> MKELIYIEEPKILFAHGQKCTDARDGLALFGPLNNLYGIKSGVIGTKQGLKIFRDYLDHIQKPIYNSNSITRPMFPGFEAVFDCKWESTGITFKEVTNEDIGKFLYNSSTHKRTYDLVSLFIDKIISANKNEDENVDVWFVIVPDEIYKYCRPNSVLPKEMVQTKALMSKSKAKSFRYEPSLFPDI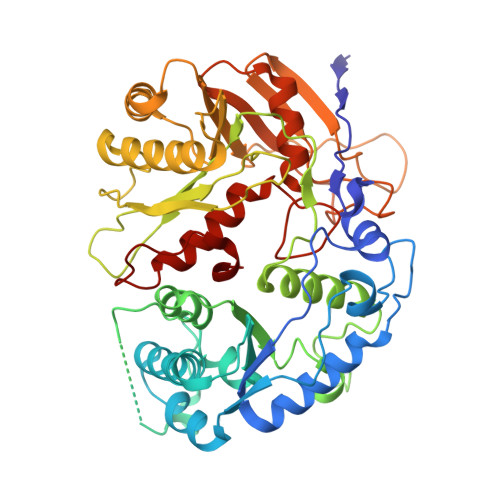NIELKEQEKEAETYNYDAQFHDQFKARLLKHTIPTQIFRESTLAWRDFKNAFGLPIRDFSKIEGHLAWTISTAAFYKAGGKPWKLSDVRNGVCYLGLVYKKVEKSKNPRNACCAAQMFLDNGDGTVFKGEVGPWYNPKNGQYHLEPKEAKALLSQSLQSYKEQIGEYPKEVFIHAKTRFNHQEWDAFLEVTPKETNLVGVTISKTKPLKLYKTEGDYTILRGNAYVVNERSAFLWTVGYVPKIQTALSMEVPNPLFIEINKGEADIKQVLKDILSLTKLNYNACIFADGEPVTLRFADKIGEILTASTDIKTPPLAFKYYI>[2x]MVHYKLTYFAIRGAGECAR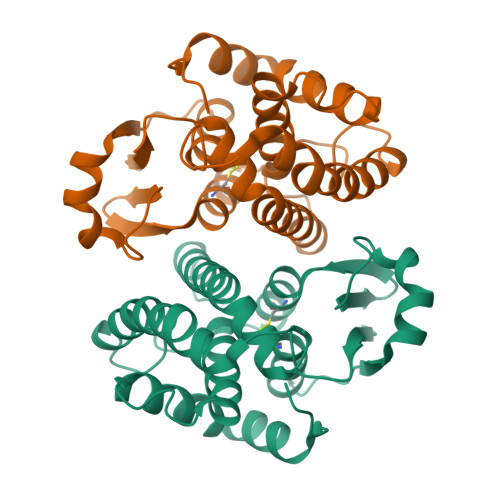QIFALADQEFEDVRLDKEQFAKVKPDLPFGQVPVLEVDGKQLAQSLAICRYLARQFGFAGKSTFDEAVVDSLADQYSDYRVEIKSFFYTVIGMREGDVEQLKKEVLLPARDKFFGFITKFLKKSPSGFLVGDSLTWVDLLVSEHNATMLTFVPEFLEGYPEVKEHMEKIRAIPKLKKWIETRPETLF~{N}-[(3~{S})-1,1-bis(oxidanylidene)thian-3-yl]-2-methyl-pyridin-3-amine | C11 H16 N2 O2 S | 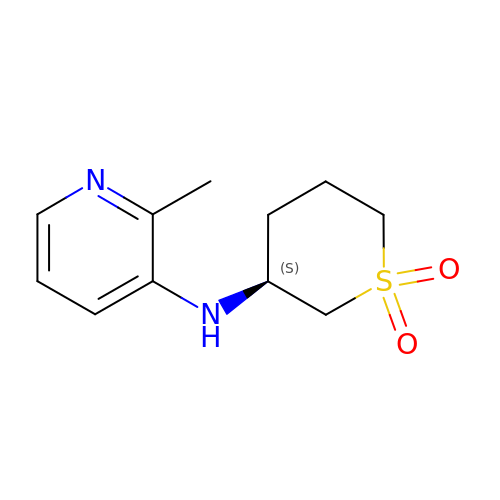UTGFIRRMSACIPX-JTQLQIEISA-N>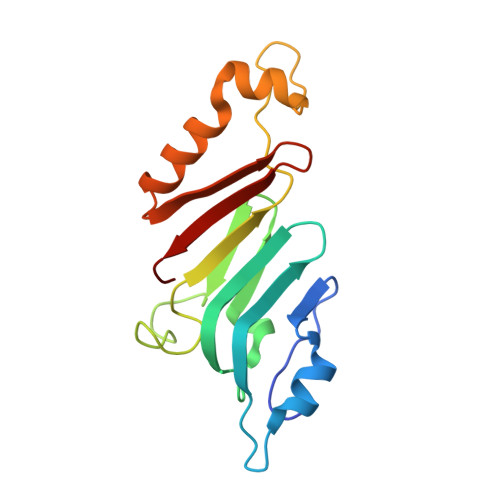 GPHMAGIILTKVGYYTIPSMDDLAKITNEKGECIVSDFTIGRKGYGSIYFEGDVNLTNLNLDDIVHIRRKEVVVYLDDNQKPPVGEGLNRKAEVTLDGVWPTDKTSRCLIKSPDRLADINYEGRLEAVSRKQGAQFKEYRPETGSWVFKVSHF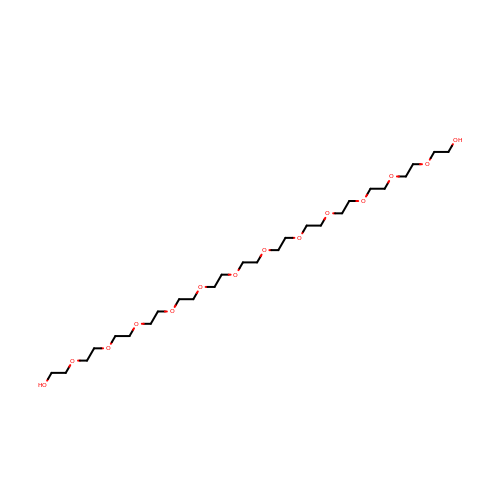3,6,9,12,15,18,21,24,27,30,33,36-dodecaoxaoctatriacontane-1,38-diol | C26 H54 O14 | AKWFJQNBHYVIPY-UHFFFAOYSA-N5-Chloro-thiophene-2-carboxylic acid 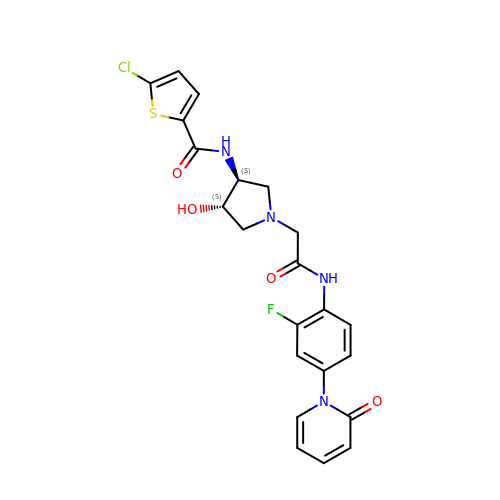((3S,4S)-1-{[2-fluoro-4-(2-oxo-2H-pyridin-1-yl)-phenylcarbamoyl]-methyl}-4-hydroxy-pyrrolidin-3-yl)-amide | C22 H20 Cl F N4 O4 S | ARAVOODWJJJNBY-IRXDYDNUSA-N> SGSEFMGEVKSVKVDNWGVFFLQKLQNFFNKTDYCDLTLQFRDNSQLKVHRLVLSACTDYFNVLEQTCEIVDDA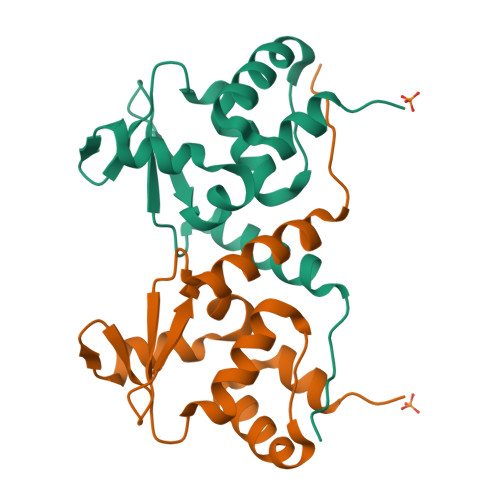LIMPNEFQADVVVPIVNFMYTGTLEFELKMYGKLLRTAKEMNMTVLLKLLEAHRRTM>GPGLNSAKEMKPFPQQVNYAGVIKPNHVTQESLNASVRSYYDNWKKKYLKNDLSSLPGGYYVKGEITGDADGFKPLGTSEGQGYGMIITVLMAGYDSNAQKIYDGLFKTARTFKSSQNPNLMGWVVADSKKAQGHFDSATDGDLDIAYSLLLAHKQWGSNGTVNYLKEAQDMITKGIKASNVTNNNQLNLGDWDSKSSLDTRPSDWMMSHLRAFYEFTGDKTWLTVINNLYDVYTQFSNKYSPNTGLISDFVVKNPPQPAPKDFLDESEYTNAYYYNASRVPLRIVMDYAMYGEKRSKVISDKVSSWIQNKTNGNPSKIVDGYQLNGSNIGSYPTAVFVSPFIAASITSSNNQKWVNSGWDWMKNKRERYFSDSYNLLTMLFITG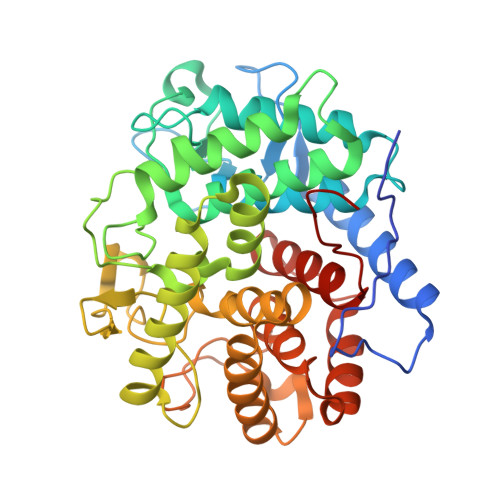NWWKPVPDDTK[2x]> SGSAGNGLVPSDPVLAETM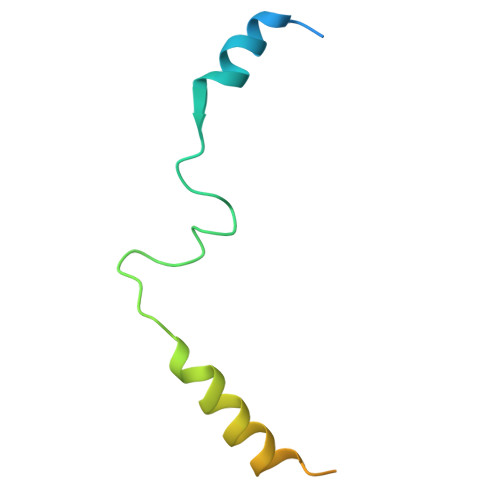KNERVVQDHNSALRGARPINFGYLIKDAELKLVQSIKGSLRGSKLPPGHKGAHGRVSKTNGS> EEKDEEFPEQKAGEVINQPMMMAARQLHDEARKWSSKGNDII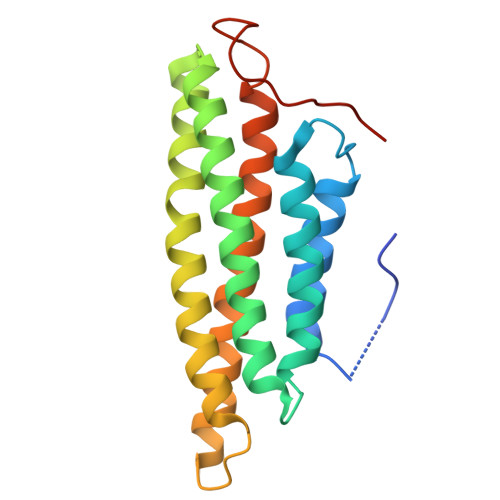AAAKRMALLMAEMSRLVRGGSGTKRALIQCAKDIAKASDEVTRLAKEVAKQCTDKRIRTNLLQVCERIPTISTQLKILSTVKATMLGRTNISDEESEQATEMLVHNAQNLMQSVKETVREAEAASIKIRTDAGFTLRWVRKTPWYQ>TRDQNGTWEMESNENFEGWMKALDIDFATRKIAVRLTLTLVIDQDGDNFKVKTTSTFYNYDVDFTVGVEFDEYTKSLDNRHVKALVTWEGDVLVCVQKGEKE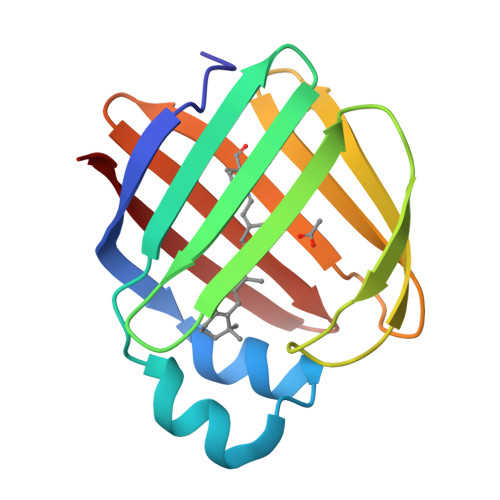NRGWKKWIEGDKLYLELTCGDQVCRQVFKKK[2x]p-Bromophenacyl bromide 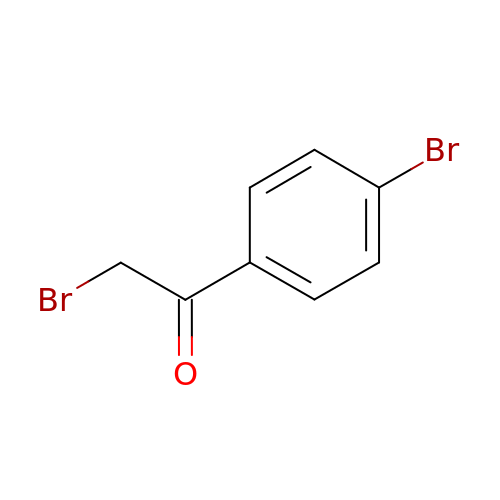| C8 H6 Br2 O | FKJSFKCZZIXQIP-UHFFFAOYSA-N>MSTAIVTNVKHFGGMGSALRLSEAGHTVA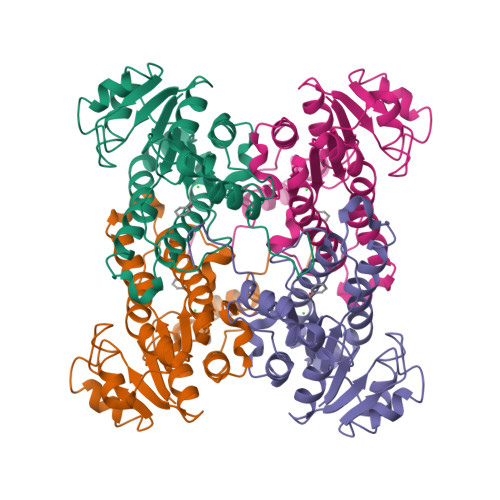CHDESFKQKDELEAFAETYPQLKPMSEQEPAELIEAVTSAYGQVDVLVSNDIFAPEFQPIDKYAVEDYRGAVEALQIRPFALVNAVASQMKKRKSGHIIFITSATPFGPWKELSTYTSARAGACTLANALSKELGEYNIPVFAIGPNYLHSEDSPYFYPTEPWKTNPEHVAHVKKVTALQRLGTQKELGELVAFLASGSCDYLTGQVFWLAGGFPMIERWPGMPE[2x]> MNQNLLVTKRDGSTERINLDKIHRVLDWAAEGLHNVSISQVELRSHIQFYDGIKTSDIHETI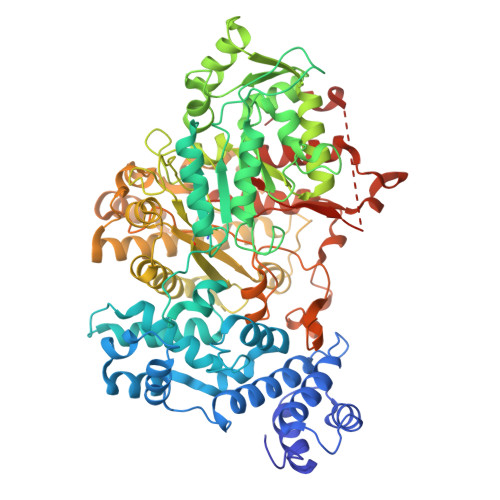IKAAADLISRDAPDYQYLAARLAIFHLRKKAYGQFEPPALYDHVVKMVEMGKYDNHLLEDYTEEEFKQMDTFIDHDRDMTFSYAAVKQLEGKYLVQNRVTGEIYESAQFLYILVAACLFSNYPRETRLQYVKRFYDAVSTFKISLPTPIMSGVRTPTRQFSSCVLIECGDSLDSINATSSAIVKYVSQRAGIGINAGRIRALGSPIRGGEAFHTGCIPFYKHFQTAVKSCSQGGVRGGAATLFYPMWHLEVESLLVLKNNRGVEGNRVRHMDYGVQINKLMYTRLLKGEDITLFSPSDVPGLYDAFFADQEEFERLYTKYEKDDSIRKQRVKAVELFSLMMQERASTGRIYIQNVDHCNTHSPFDPAIAPVRQSNLCLEIALPTKPLNDVNDENGEIALCTLSAFNLGAINNLDELDELAILAVRALDALLDYQDYPIPAAKRGAMGRRTLGIGVINFAYYLAKHGKRYSDGSANNLTHKTFEAIQYYLLKASNELAKEQGACPWFNETTYAKGILPIDTYKKDLDTIANEPLHYDWEALRESIKTHGLRNSTLSALMPSETSSQISNATNGIEPPRGYVSIKASKDGILRQVVPDYEHLHDAYELLWEMPGNDGYLQLVGIMQKFIDQSISANTNYDPSRFPSGKVPMQQLLKDLLTAYKFGVKTLYYQNTRDDIDDLSNFQLPSIQDDGCESGACKI>MWSHPQFEKGGSSGGVDMKGPNLNFRKTPSKDNGVKQVESLARPETPPPKFVEDSNLEFNVLASEKLPNYTNLDLFHRAVFPFMFLAQCVAIMPLVGIRESNPRRVRFAYKSIPMFVTLIFMIATSILFLSMFTHLLKIGITAKNFVGLVFFGCVLSAYVVFIRLAKKWPAVVRIWTRTEIPFTKPPYEIPKRNLSRRVQLAALAIIGLSLGEHALYQVSAILSYTRRIQMCANITTVPSFNNYMQTNYDYVFQLLPYSPIIAVLILLINGACTFVWNYMDLFIMMISKGLSYRFEQITTRIRKLEHEEVCESVFIQIREHYVKMCELLEFVDSAMSSLILLSCVNNLYFVCYQLLNVFNKLRWPINYIYFWYSLLYLIGRTAFVFLTAADINEESKRGLGVLRRVSSRSWCVEVERLIFQMTTQTVALSGKKFYFLTRRLL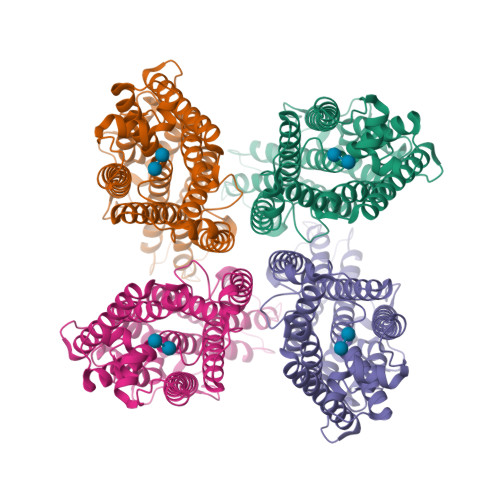FGMAGTIVTYELVLLQFDEPNRRKGLQPLCA[4x]> MALKGNMQVENLEAVEDPQVDLGAQVSAAPRAKRQARQAEDVQGEDPYLESISELDDVLLKFKKYSKSMSSIENKVFSSSSGCFKSKNERVDAYSFACSSYTDKIEEYLYDPANSFPYKRGVKLVPKE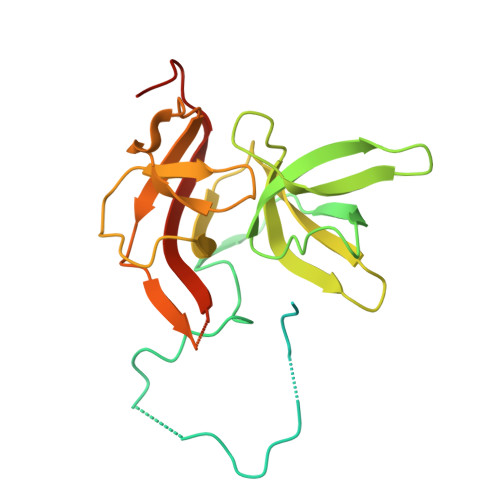NSIYVEVGADTDMYGICVDVCEFSCTAYVLPITNNFEGYLVTRNPSIKIGEILDINNNGVIIKAGGGPPTAINIYALSDSFTINFAPEDGNQDQNRYPRQEYSINLIKVAIFGNRGLEKTVNPDGG> DITVYNGQHKEAATAVAKAFEQETGIKVTLNSGKSEQLAGQLKEEGDKTPADVFYTEQTATFADLSEAGLLAPISEQTIQQTAQKGVPLAPKKDWIALSGRSRVVVYDHTKLSE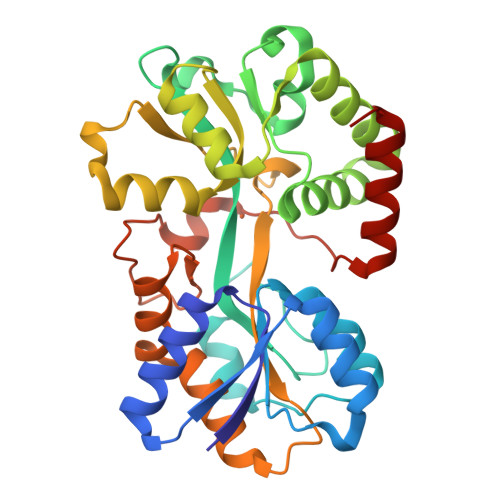KDMEKSVLDYATPKWKGKIGYVSTSGAFLEQVVALSKMKGDKVALNWLKGLKENGKLYAKNSVALQAVENGEVPAALILNYYWYNLAKEKGVENLKSRLYFVRHQDPGALVSYSGAAVLKASKNQAEAQKFVDFLASKKGQEALVAARAEYPLRADVVSPFNLEPYEKLEAPVVSATTAQDKEHAIKLIEEAGLK> ETYSVDSPGLYITEFKVDDLSRHYVLDPGLEFYYNHYYRILLFVNKVYVGPLIGPIDITRYLKPGVNEVALLVEWGVVNPVIGVYQYKVDGEWFIQEGLHGLIEEWFRRSPRGETAEPPILLGDKAGRVIWVNTVIPYEKEPTSSSPVKLEVDFWG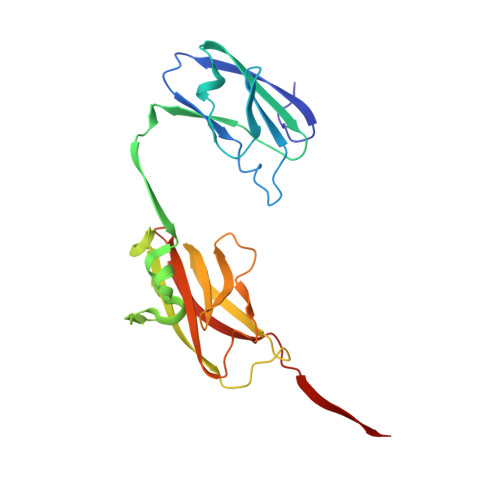CRILVFVNGEFIGRISDDSPERELYVPETAVRRGLNNITLLAIVTSRSSGIRGLRLKETYVHERKEIVFKL>MSKRPNFLVIVADDLGFSDIGAFGGEIATPNLDALAIAGLRLTDFHTASAASPTRSMLLTGTDHHIAGIGTVAEALTPELEGKPGYEGHLNERVVALPELLREAGYQTLMAGKWHLGLKPEQTPHARGFERSFSLLPGAANHYGFEPPYDESTPRILKGTPALYVEDERYLDTLPEGFYSSDAFGDKLLQYLKERDQSRPFFAYLPFSAPHWPLQAPREIVEKYRGRYDAGPEALRQERLARLKELGLVEADVEAHPVLALTREWEALEDEERAKSARAMEVYAAMVERMDWNIGRVVDYLRRQGELDNTFVLFMSDNGAEGALLEAFPKFGPDLLDFLDRHYDNSLENIGSANSYVWYGPRWAQAATAPSRLYKAFTTQGGIRVPALVRYPRLSRQGAISHAFATVMDVTPTLLDLAGVRHPGKRWRGREIAEPRGRSWLGWLSGETEAAHDENTVTGWGLFGMRAIRQGDWKAVYLPAPVGPATWQLYDLAR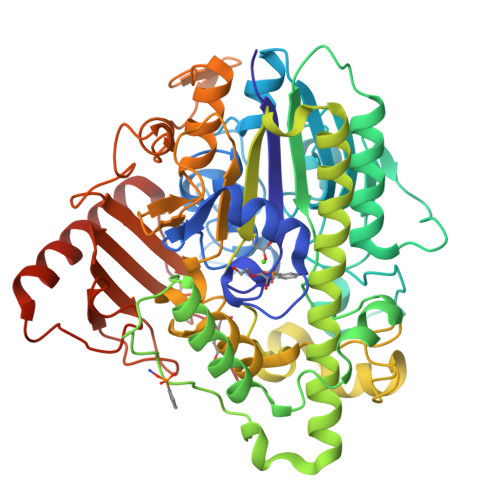DPGEIHDLADSQPGKLAELIEHWKRYVSDTGVVEGASPFLVR[2x]[(2~{S})-3-[[(1~{S})-1-(3,4-dichlorophenyl)ethyl]amino]-2-oxidanyl-propyl]-(phenylmethyl)phosphinic acid | C18 H22 Cl2 N O3 P | 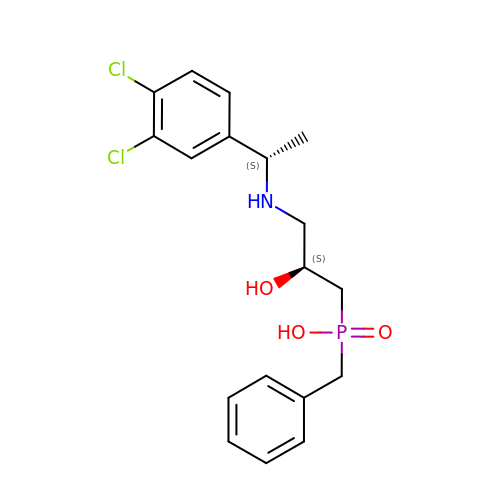ZODSPDOOCZZEIM-BBRMVZONSA-N> MYSKIKISGTIEVVTGLHIGGGGESSMIGAIDSPVVRDLQTKLPIIPGSSIKGKMRNLLAKHFGLKMKQESHNQDDERVLRLFGSSEKGNIQR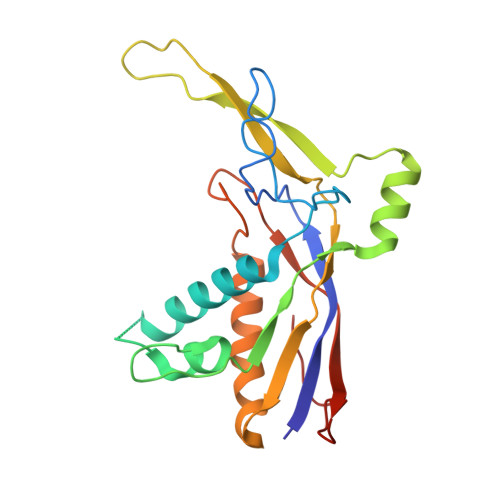ARLQISDAFFSEKTKEHFAQNDIAYTETKFENTINRLTAVANPRQIERVTRGSEFDFVFIYNVDEESQVEDDFENIEKAIHLLENDYLGGGGTRGNGRIQFKDTNIETVVGEYDSTNLKIK>MSLASYFIGVDVGTGSARAGVFDLQGRMVGQASREITMFKPKADFVEQSSENIWQAVCNAVRDAVNQADINPIQVKGLGFDATCSLVVLDKEGNPLTVSPSGRNEQNVIVWMDHRAITQAERINATKHPVLEFVGGVISPEMQTPKLLWLKQHMPNTWSNVGHLFDLPDFLTWR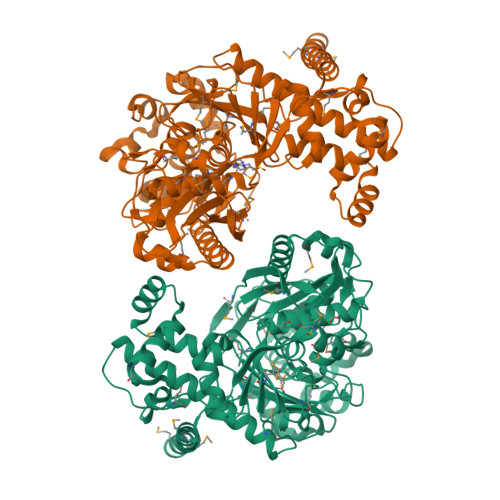ATKDETRSLCSTVCKWTYLGHEDRWDPSYFKLVGLADLLDNNAAKIGATVKPMGAPLGHGLSQRAASEMGLIPGTAVSVSIIDAHAGTIGILGASGVTGENANFDRRIALIGGTSTAHMAMSRSAHFISGIWGPYYSAILPEYWLNEGGQSATGALIDHIIQSHPCYPALLEQAKNKGETIYEALNYILRQMAGEPENIAFLTNDIHMLPYFHGNRSPRANPNLTGIITGLKLSTTPEDMALRYLATIQALALGTRHIIETMNQNGYNIDTMMASGGGTKNPIFVQEHANATGCAMLLPEESEAMLLGSAMMGTVAAGVFESLPEAMAAMSRIGKTVTPQTNKIKAYYDRKYRVFHQMYHDHMRYQALMQEGEGHHHHHH[2x]Sarcosine oxidase from Bacillus sp. (SoxB) recognizes the cyclic imino acids l‐proline (l‐Pro), d‐proline (d‐Pro), and l‐thioproline (l‐Tpr) as minor substrates.

The reaction behavior varied depending on the substrates; notably, the absorption spectrum of l‐Tpr exhibited charge transfer, which was characteristic of substrate inhibition. Crystal structures of the enzyme–substrate complexes suggested that Tyr254 causes spatial interference with cyclic imino acids at the active site. A water network was also identified near the enzyme's active site, interacting with the side chain of Tyr254.

>[2x]STHFDVIVVGAGSMGMAAGYQLAKQGVKTLLVDAFDPPHTNGSHHGDTRIIRHAYGEGREYVPLALRSQELWYELEKETHHKIFTKTGVLVFGPKGESAFVAETMEAAKEHSLTVDLLEGDEINKRWPGITVPENYNAIFEPNSGVLFSENCIRAYRELAEARGAKVLTHTRVEDFDISPDSVKIETANGSYTADKLIVSMGAWNSKLLSKLNLDIPLQPYRQVVGFFESDESKYSNDIDFPGFMVEVPNGIYYGFPSFGGCGLKLGYHTFGQKIDPDTINREFGVYPEDESNLRAFLEEYMPGANGELKRGAVCMYTKTLDEHFIIDLHPEHSNVVIAAGFSGHGFKFSSGVGEVLSQLALTGKTEHDISIFSINRPALKESLQKTTIGSHHHHHH>KPGAPWWKSAVFYQVYPRSFKDTNGDGIGDFKGLTEKLDYLKGLGIDAIWINPHYASPNTDNGYDISDYREVMKEYGTMEDFDRLMAELKKRGMRLMVDVVINHSSDQHEWFKSSRASKDNPYRDYYFWRDGKDGHEPNNYPSFFGGSAWEKDPVTGQYYLHYLGRQQPDLNWDTPKLREELYAMLRFWLDKGVSGMRFDTVATYSKTPGFPDLTPEQMKNFAEAYTQGPNLHRYLQEMHEKVFDHYDAVTAGEIFGAPLNQVPLFIDSRRKELDMAFTFDLIRYDRALDRWHTIPRTLADFRQTIDKVDAIAGEYGWNTFFLGNHDNPRAVSHFGDDRPQWREASAKALATVTLTQRGTPFIFQGDELGMTNYPFKTLQDFDDIEVKGFFQDYVETGKATAEELLTNVALTSRDNARTPFQWDDSANAGFTTGKPWLKVNPNYTE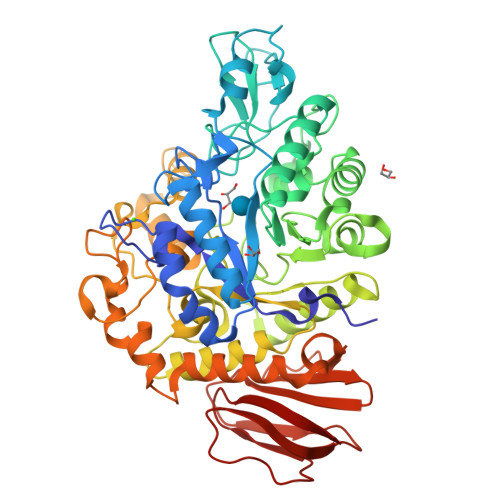INAAREIGDPKSVYSFYRNLISIRHETPALSTGSYRDIDPSNADVYAYTRSQDGETYLVVVNFKAEPRSFTLPDGMHIAETLIESSSPAAPAAGAASLELQPWQSGIYKVK[2x]> DPTDLSFSPDEINKLIETGLNTVEYFT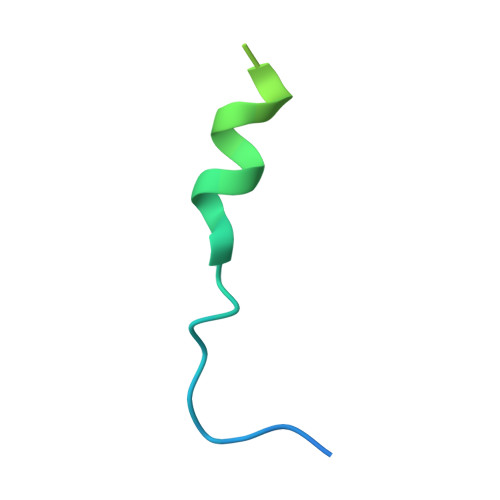SQQVTGTSSLGKNTIPPGVTGL> SNAMILPSFPDLTGLVVNLKFTARAEFSLNHEMAVDAFLRHS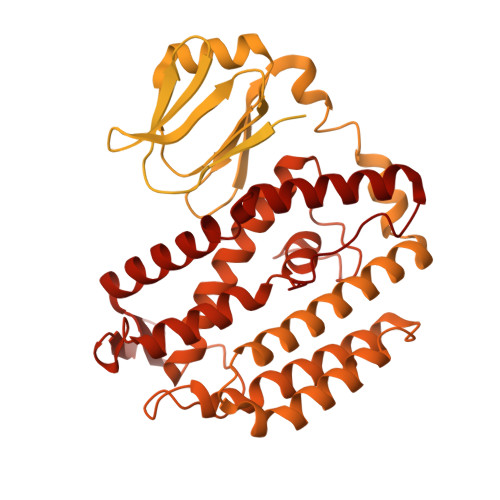LNLGESYSHHLSIITPENGRLFYREGDTYRFVVIAMGNQQQTNSIWHTLINHLRKLPDSAPITDKQAPLRNNIKLESLNDLFDGIPVSSKESLDAYTLQRAMEQGLAWHKAANLTEQPLDIQWYWQSTVRILHADHKQHKGEQRYCRDAVQLTPLLLLKRIYETLNNVATYFGLKTNKNTTENHQAWLKEQAQYIEIQHPDLYWIDTPYFGKDAEKNTLGGMAGNFTLSLKPGIEPGLLAMLILTQMVGVGQRRTSGLGKYWLKHSLKHAHLILGLKPNRVTRSQTLLDCIIQPHIISQAIAEIEKKTNIDTLNERTLSQVQSAIGQLRKHQYQAPKLQGFTIPKKDGTERLLAVSPLYDRILQKAAAIVLTPGLDAIMSQASYGYRKGLSRQQVRYEIQNAYRQGYHWVYESDIEDFFDAVYRPQLINRLKSLLGNDPLWEQIESWLGQDIHIKDTIIERTPNLGLPQGSPLSPLLANFILDDFDSDLETHGFKIIRFADDFIILCKSQHEAQQAAHAVEQSLKEVKLSINVEKTHIIQLNQGFRFLGYLFREDHAIEIAGEKSDGRTTFAAEQTPTNLPPWLANLGTKSPQPLADDDLPKKSYGQIETQGTHLVLAGDAQIITTDNQNLIVKKDDKITHKISLEQLHAVTLIGLHTMTLPAKHRLLEHKIPVHIADRTGRYLGAVTSFQPAQNNYKNWFIQLQMCDREPFAHAIAQQIVISRIHNQRQTLLKRKAHRKQLQQTLSNLKKLQYKVTAATKRSSLNGLEGSATREYFQQFNLFLPEWAHFSKRTRRPPKDPFNVLLSLGYTILYSHTDAILQSAGFITWKGIYHQQSAAHAALASDIMESYRHLVERYAIYIINHGQIKQDDFRQEKDHLGQDTIRLSAEARRRYVGGLINRFQKFSKDKTLHQHLYQQAQQLKNAMHNQQSSQFQVWKELK>[2x]QEVEFDIPPQALGSALQEFGRQADIQVLYRPEEVRNKRSSAIKGKLEPNQAITELLRGTGASVDFQGNAITISVAEAADSSVDLGATMITSNQLGTITEDSGSYTPGTIATATRLVLTPRETPQSITVVTRQNMDDFGLNNIDDVMRHTPGITVSAYDTDRNNYYARGFSINNFQYDGIPSTARNVGY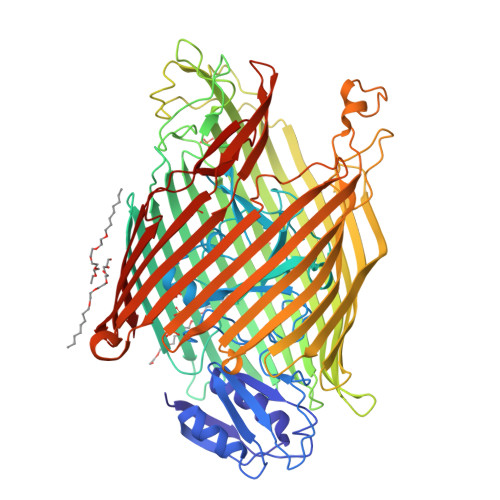SAGNTLSDMAIYDRVEVLKGATGLLTGAGSLGATINLIRKKPTHEFKGHVELGAGSWDNYRSELDVSGPLTESGNVRGRAVAAYQDKHSFMDHYERKTSVYYGILEFDLNPDTMLTVGADYQDNDPKGSGWSGSFPLFDSQGNRNDVSRSFNNGAKWSSWEQYTRTVFANLEHNFANGWVGKVQLDHKINGYHAPLGAIMGDWPAPDNSAKIVAQKYTGETKSNSLDIYLTGPFQFLGREHELVVGTSASFSHWEGKSYWNLRNYDNTTDDFINWDGDIGKPDWGTPSQYIDDKTRQLGSYMTARFNVTDDLNLFLGGRVVDYRVTGLNPTIRESGRFIPYVGAVYDLNDTYSVYASYTDIFMPQDSWYRDSSNKLLEPDEGQNYEIGIKGEYLDGRLNTSLAYFEIHEENRAEEDALYNSKPTNPAITYAYKGIKAKTKGYEAEISGELAPGWQVQAGYTHKIIRDDSGKKVSTWEPQDQLSLYTSYKFKGALDKLTVGGGARWQGKSWQMVYNNPRSRWEKFSQEDYWLVDLMARYQITDKLSASVNVNNVFDKTYYTNIGFYTSASYGDPRNLMFSTRWDF;> SAKQQKG> MSLTFPTLSPTQIIQYIHLGSFLNAHNVDYIHNNNISSILLVGIEVPSLFKDQCDILRLDIVSEEGHQLYDSIPNAIKFIIRSIQRKEGVLIISGTGV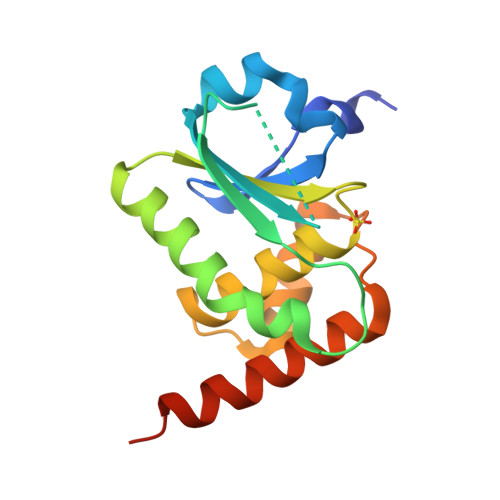NKAPAIVIAFLMYYQRLSFINAFNKVQGLYPLIDIESGFILQLKLFEKKLEKMNSEGHHHHHH Eukaryotes have two types of DNA clamps: the replication clamp PCNA and the checkpoint clamp RAD9-RAD1-HUS1 (9-1-1). 9-1-1 activates the ATR-CHK1 pathway in DNA damage checkpoint, regulating cell cycle progression. Structure of 9-1-1 consists of two moieties: a hetero-trimeric ring formed by PCNA-like domains of three subunits and an intrinsically disordered C-terminal region of the RAD9 subunit, called RAD9 C-tail. In contrast, RHINO, a 9-1-1 binding protein, interacts with both RAD1 and RAD9 subunits, positively regulating checkpoint activation by 9-1-1.

Assuming that hydrophobic or aromatic residues of RHINO are involved in interactions with RAD9, a conserved region of RHINO (88-TSKFPHLTFESP-99) was considered a candidate peptide binding to the hydrophobic pocket of RAD9. Crystallization trials of the 9-1-1 ring in the presence of the RHINO peptide were performed, and crystals suitable for X-ray diffraction study were successfully obtained. Ultimately, the crystal structure of the 9-1-1 ring in complex with the RHINO peptide was determined at 2.81 Å resolution. In contrast to the RAD1-binding region of RHINO, which binds to the edge-to-back side of the RAD1 subunit, the RHINO peptide (residues 88–99) binds to the hydrophobic pocket on the front side of RAD9, across the IDC-loop of RAD9. The hydrophobic pocket consists of two binding sites, subsite-1 and subsite-2. RHINO bound to RAD9 adopts an extended conformation, distinct from the PIP-box that forms a helical conformation upon binding to PCNA. The side-chain of Phe91 of RHINO is accommodated into the subsite-1, and the side-chains of Leu94 and Phe96 of RHINO are accommodated into the subsite-2. These side-chains interact with residues in these subsites through vdW contacts. Hydrogen bonding interactions through main-chains are also observed in the crystal structure, where the main-chains of Leu94, Thr95, and Glu97 of RHINO form hydrogen bonds with the main-chains of Arg45, Val135, and Gln133 of RAD9, respectively. Phe91, Leu94, and Phe96 of RHINO correspond to Phe361, Leu364, and Phe366 of RAD9, respectively, suggesting that interactions of RAD9 C-tail with RAD9 could be similar to those observed in the present structure. The biochemical and structural analysis revealed the mechanisms underlying intra- and inter-molecular interactions on RAD9, suggesting that the representative sequence for binding to RAD9 would be FxxLxF.

> MKCLVTGGNVKVLGKAVHSLSRIGDELYLEPLEDGLSLRTVNSSRSAYACFLFAPLFFQQYQAATPGQDLLRCKILMKSFLSVFRSLAMLEKTVEKCCISLNGRSSRLVVQLHCKFGVRKTHNLSFQDCESLQAVFDPASCPHMLRAPARVLGEAVLPFSPALAEVTLGIGRGRRVILRSYHEEEADSTAKAMVTEMCLGEEDFQQLQAQEGVAITFCLKEFRGLLSFAESANLNLSIHFDAPGRPAIFTIKDSLLDGHFVLATLSDTDS;> MHHHHHHKFRAKIVDGACLNHFTRISNMIAKLAKTCTLRISPDKLNFILCDKLANGGVSMWCELEQENFFNEFQMEGVSAENNEIYLELTSENLSRALKTAQNARALKIKLTNKHFPCLTVSVELLSMSSSSRIVTHDIPIKVIPRKLWKDLQEPVVPDPDVSIYLPVLKTMKSVVEKMKNISNHLVIEANLDGELNLKIETELVCVTTHFKDLGNPPLASESTHEDRNVEHMAEVHIDIRKLLQFLAGQQVNPTKALCNIVNNKMVHFDLLHEDVSLQYFIPALS;> MPLLTQQIQDEDDQYSLVASLDNVRNLSTILKAIHFREHATCFATKNGIKVTVENAKCVQANAAIQAGIFQEFKVQEESVTFRINLTVLLDCLSIFGSSPMPGTLTALRMCYQGYGYPLMLFLEEGGVVTVCKINTQEPEETLDFDFCSTNVINKIILQSEGLREAFSELDMTSEVLQITMSPDKPYFRLSTFGNAGSSHLDYPKDSDLMEAFHCNQTQVNRYKISLLKPSTKALVLSCKVSIRTDNRGFLSLQYAIRNEDGQICAVEYYCCPDEEVPESES;> TSKFPHLTFESP> MELQQNFTDNNSIKYTAILILIAFAFSVLARLYWVAWASEFYEFFFNDQLMITTNDGYAFAEGARDMIAGFHQPNDLSYFGSSLSTLTYWLYSILPFSFESIILYMSTFFASLIVVPIILIAREYKLTTYGFIAALLGSIANSYYNRTMSGYYDTDMLVLVLPMLILLTFIRLTINKDIFTLLLSPVFIMIYLWWYPSSYSLNFAMIGLFGLYTLVFHRKEKIFYLTIALMIIALSMLAWQYKLALIVLLFAIFAFKEEKINFYMIWALIFISILILHLSGGLDPVLYQLKFYVFKASDVQNLKDAAFMYFNVNETIMEVNTIDPEVFMQRISSSVLVFILSFIGFILLLKDHKSMLLALPMLALGFMALRAGLRFTIYAVPVMALGFGYFLYAFFNFLEKKQIKLSLRNKNILLILIAFFSISPALMHIYYYKSSTVFTSYEASILNDLKNKAQREDYVVAWWDYGYPIRYYSDVKTLIDGGKHLGKDNFFSSFVLSKEQIPAANMARLSVEYTEKSFKENYPDVLKAMVKDYQKTSAKDFLESLNDPNFKIDTPKTRDVYIYMPYRMLRIMPVVAQFANTNPDNGEQEKSLFFSQANPLDQDKKQGSITLDNGVEISNDYRSLKIEGNSIPLKAFVDIESITNGKFYYNEIDSKAQIYLLYLREYKSYVILDESLYNSSYIQMFLLNQYDQDLFEQITNDTRAKIYRLKREFHHHHHHHHHH;> GDQAATFG

N-protein glycosylation is a post-translational modification that is conserved in all domains of life. The oligosaccharide is first assembled on a pyrophosphate-lipid carrier and then transferred en bloc to conserved sequons (N-X-S/T) of secretory proteins. The reaction is catalyzed by an integral-membrane oligosaccharyltransferase (OST). X-ray structures of ssOSTs of Campylobacter lari (PglB) and Archaeoglobus fulgidus (AglB) have revealed the fold of the enzyme.

Here we present the X-ray structure of PglB in complex with an inhibitory peptide and a synthetic reactive LLO analog. We chose 2,4-diaminobutanoic acid (Dab) to replace the acceptor asparagine, because Dab-containing peptides were previously shown to act as competitive inhibitors of bacterial and eukaryotic OSTs at physiological pH. We used the reactive synthetic LLO analog ωZZZ-PP-GlcNAc, which is chemically very similar to the wild type LLO except that it contains a GlcNAc rather than di-N-acetyl-bacillosamine as a reducing-end sugar. The key difference is that the two substrates are closer in the new ternary complex, with a distance of ~3.4 Å between carbon C-1 of the GlcNAc moiety of reactive LLO and the –NH2 group of the Dab residue, representative of the atoms that would form an N-glycosidic bond if Dab was replaced by Asn. Whereas the lipid tail of the LLO analog has an indistinguishable conformation to the previous ternary complex, the pyrophosphate and GlcNAc moieties have shifted and interact differently with the surface of PglB in the new structure. We now observe continuous electron density between the pyrophosphate group of LLO and the catalytic Mn2+, with the shortest distance (~4  Å) observed between Mn2+ and the oxygen linking C1 of GlcNAc and the pyrophosphate moiety. The structure also revealed different interactions between the pyrophosphate of the LLO and two essential catalytic residues, R375 and Y196. In the present structure, the N-acetyl group can form hydrogen bonds with the side chains of both D56 and Y468. The Dab side chain reaches the catalytic site where it can form hydrogen bonds with three conserved and catalytically essential residues, the side chains of D56 and E319 and the main chain carbonyl oxygen of G482.>MSQDNNYSQGPVPISARKGGLALTFVMLGLTFFSASMWTGGALGTGLSFNDFFLAVLIGNLLLGIYTAFLGFIGSKTGLTTHLLARYSFGIKGSWLPSFLLGGTQVGWFGVGVAMFAIPVGKATGIDINLLIAVSGILMTITVFFGISALTVLSIIAVPAIAILGSYSVYLAIHDMGGLSTLMNVKPTQPLDFNLALAMVVGSFISAGTLTADFVRFGRNPKVAVVVAIIAFFLGNTLMFVFGAAGAASLGMADISDVMIAQGLLLPAIVVLGLNIWTTNDNALYASGLGFANITGLSSKKLSVINGIVGTVCALWLYNNFVGWLTFLSAAIPPVGGVIIADYLMNKARYNTFNIATMQSVNWVALLAVAIGIVAGHWLPGIVPVNAVLGGAISYAVLNPILNRRTARQAEISHAGSLEVLFQ[2x]

CodB is a cytosine transporter from the Nucleobase‐Cation‐Symport‐1 (NCS1) transporter family, a member of the widespread LeuT superfamily. Members of the family are responsible for transporting nucleobases and related molecules into cells, often as components of salvage pathways. We show that CodB carries out the sodium‐dependent uptake of cytosine and can bind 5‐fluorocytosine. The overall 12‐TM helix topology is very similar to Mhp1: TM1‐TM5 are related to TM6‐TM10 by a pseudo 2‐fold axis and intertwine to form the bundle and hash motifs.

CodB was purified and crystallised in the presence of cytosine using the lipidic cubic phase (LCP) method (Caffrey & Cherezov, 2009) and the structure was determined and refined at 2.4 Å to an Rfactor of 20.1% and a corresponding Rfree of 24.6% with excellent density. CodB crystallises as a monomer with two molecules in the asymmetric unit orientated oppositely with respect to the membrane plane. Both molecules adopt an outward‐open conformation (and EV2) with cytosine bound in a solvent accessible polar pocket and density consistent with a Na+ ion observed in the conserved Na2 site. The cytosine substrate is found at the interface of the hash‐motif and the 4‐helix bundle, sandwiched between two aromatic residues, Trp108 of TM3 of the hash domain and Phe204 of TM6 of the bundle domain in a face‐to‐face pi stacking arrangement. The cytosine forms two direct hydrogen bonds to the main chain at either side of the breakpoint of TM6 of the bundle domain: to the carbonyl oxygen of Ser203 of TM6a and to the main chain nitrogen atom of Ala207 of TM6b. In terms of interactions with the hash motif, as well as stacking with Trp108, there is a hydrogen bond from the cytosine to the amino oxygen of Gln105 of TM3 and a potential water‐mediated hydrogen bond to Asn280 of TM8. The sodium ion is coordinated by the main chain carbonyl oxygens of Gly29 and Phe32 at the breakpoint of TM1 of the bundle domain and the main chain carbonyl oxygen of Asn275 and the hydroxyl oxygens of Thr278 and Thr279 from TM8 of the hash domain in a square pyramidal arrangement. In an unusual interaction that is not seen in other Na+‐coupled LeuT members, the side chain of Asn275 is also within hydrogen‐bond distance of the side chain hydroxyl and the amide nitrogen of Ser34 at the C‐terminus of TM1b, providing a further link between the hash and bundle domains when sodium binds. Between EL4 and the tip of TM3, TM10 and TM1 there is non‐protein density, which we have tentatively modelled as DDM and monoolein respectively (Fig EV2). Although TM10 in CodB is one residue shorter than in Mhp1, given that the temperature factors are high for TM10 and the helix retains the proline on TM10 around which TM10 swivels it seems likely that the lipid‐like molecules that we observe in the density are preventing the conformation adopted in the substrate‐bound form of Mhp1 rather than a substantial difference in mechanism.>[2x]MAHHHHHHHHHHGSTSGSGEQKLISEEDLGSTSGSGDYKDDDDKLTSLYKKAGLENLYFQGMAQSRQLFLFGDQTADFVPKLRSLLSVQDSPILAAFLDQSHYVVRAQMLQSMNTVDHKLARTADLRQMVQKYVDGKLTPAFRTALVCLCQLGCFIREYEESGNMYPQPSDSYVLGFCMGSLAAVAVSCSRSLSELLPIAVQTVLIAFRLGLCALEMRDRVDGCSDDRGDPWSTIVWGLDPQQARDQIEVFCRTTNVPQTRRPWISCISKNAITLSGSPSTLRAFCAMPQMAQHRTAPIPICLPAHNGALFTQADITTILDTTPTTPWEQLPGQIPYISHVTGNVVQTSNYRDLIEVALSETLLEQVRLDLVETGLPRLLQSRQVKSVTIVPFLTRMNETMSNILPDSFISTETRTDTGRAIPASGRPGAGKCKLAIVSMSGRFPESPTTESFWDLLYKGLDVCKEVPRRRWDINTHVDPSGKARNKGATKWGCWLDFSGDFDPRFFGISPKEAPQMDPAQRMALMSTYEAMERAGLVPDTTPSTQRDRIGVFHGVTSNDWMETNTAQNIDTYFITGGNRGFIPGRINFCFEFAGPSYTNDTACSSSLAAIHLACNSLWRGDCDTAVAGGTNMIYTPDGHTGLDKGFFLSRTGNCKPYDDKADGYCRAEGVGTVFIKRLEDALADNDPILGVILDAKTNHSAMSESMTRPHVGAQIDNMTAALNTTGLHPNDFSYIEMHGTGTQVGDAVEMESVLSVFAPSETARKADQPLFVGSAKANVGHGEGVSGVTSLIKVLMMMQHDTIPPHCGIKPGSKINRNFPDLGARNVHIAFEPKPWPRTHTPRRVLINNFSAAGGNTALIVEDAPERHWPTEKDPRSSHIVALSAHVGASMKTNLERLHQYLLKNPHTDLAQLSYTTTARRWHYLHRVSVTGASVEEVTRKLEMAIQNGDGVSRPKSKPKILFAFTGQGSQYATMGKQVYDAYPSFREDLEKFDRLAQSHGFPSFLHVCTSPKGDVEEMAPVVVQLAITCLQMALTNLMTSFGIRPDVTVGHSLGEFAALYAAGVLSASDVVYLVGQRAELLQERCQRGTHAMLAVKATPEALSQWIQDHDCEVACINGPEDTVLSGTTKNVAEVQRAMTDNGIKCTLLKLPFAFHSAQVQPILDDFEALAQGATFAKPQLLILSPLLRTEIHEQGVVTPSYVAQHCRHTVDMAQALRSAREKGLIDDKTLVIELGPKPLISGMVKMTLGDKISTLPTLAPNKAIWPSLQKILTSVYTGGWDINWKKYHAPFASSQKVVDLPSYGWDLKDYYIPYQGDWCLHRHQQDCKCAAPGHEIKTADYQVPPESTPHRPSKLDPSKEAFPEIKTTTTLHRVVEETTKPLGATLVVETDISRKDVNGLARGHLVDGIPLCTPSFYADIAMQVGQYSMQRLRAGHPGAGAIDGLVDVSDMVVDKALVPHGKGPQLLRTTLTMEWPPKAAATTRSAKVKFATYFADGKLDTEHASCTVRFTSDAQLKSLRRSVSEYKTHIRQLHDGHAKGQFMRYNRKTGYKLMSSMARFNPDYMLLDYLVLNEAENEAASGVDFSLGSSEGTFAAHPAHVDAITQVAGFAMNANDNVDIEKQVYVNHGWDSFQIYQPLDNSKSYQVYTKMGQAKENDLVHGDVVVLDGEQIVAFFRGLTLRSVPRGALRVVLQTTVKKADRQLGFKTMPSPPPPTTTMPISPYKPANTQVSSQAIPAEATHSHTPPQPKHSPVPETAGSAPAAKGVGVSNEKLDAVMRVVSEESGIALEELTDDSNFADMGIDSLSSMVIGSRFREDLGLDLGPEFSLFIDCTTVRALKDFMLGSGDAGSGSNVEDPPPSATPGINPETDWSSSASDSIFASEDHGHSSESGADT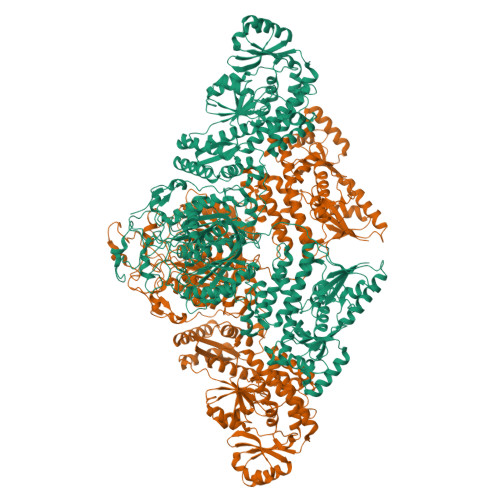GSPPALDLKPYCRPSTSVVLQGLPMVARKTLFMLPDGGGSAFSYASLPRLKSDTAVVGLNCPYARDPENMNCTHGAMIESFCNEIRRRQPRGPYHLGGWSSGGAFAYVVAEALVNQGEEVHSLIIIDAPIPQAMEQLPRAFYEHCNSIGLFATQPGASPDGSTEPPSYLIPHFTAVVDVMLDYKLAPLHARRMPKVGIVWAADTVMDERDAPKMKGMHFMIQKRTEFGPDGWDTIMPGASFDIVRADGANHFTLMQKEHVSIISDLIDRVMA4-[4-[(4,4-dimethylpiperidin-1-yl)methyl]-2-fluoranyl-phenyl]-9-[6-(methylamino)pyrimidin-4-yl]-1,4,9-triazaspiro[5.5]undecan-2-one 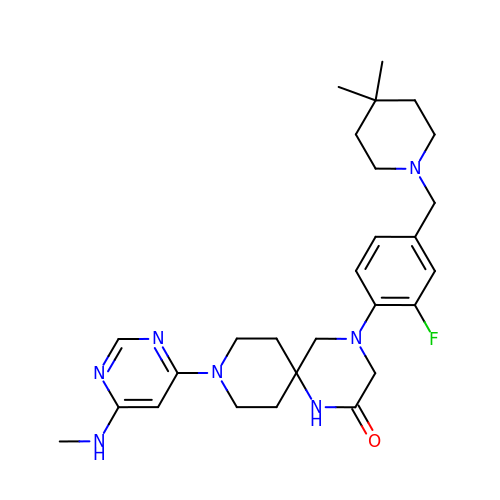| C27 H38 F N7 O | JFMKIJDUIQGGII-UHFFFAOYSA-N> MNHKVHHHHHHIEGRHMDEYKQVDVGKDGMVATAHPLASEIGADVLKKGGNAIDAAVAIQFALNVTEPMMSGIGGGGFMMVYDGKTKDTTIIDSRERAPAGATPDMF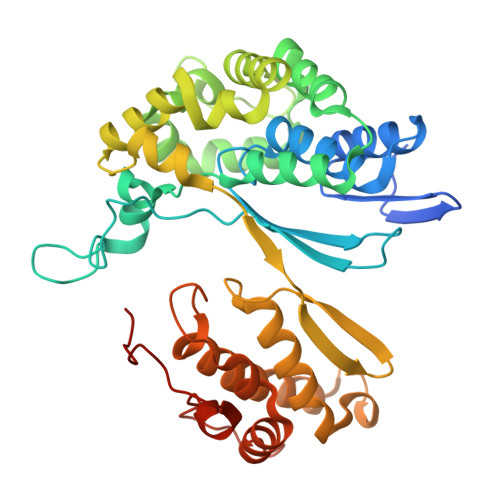LDENGKAIPFSERVTKGTAVGVPGTLKGLEEALDKWGTRSMKQLITPSIKLAEKGFPIDSVLAEAISDYQEKLSRTAAKDVFLPNGEPLKEGDTLIQKDLAKTFKLIRSKGTDAFYKGKFAKTLSDTVQDFGGSMTEKDLENYDITIDEPIWGDYQGYQIATTPPPSSGGIFLLQMLKILDHFNLSQYDVRSWEKYQLLAETMHLSYADRASYAGDPEFVNVPLKGLLHPDYIKERQQLINLDQVNKKPKAGDPWKYQEGSANYKQVEQPKDKVEGQ>[2x]GSHMPMYEVQWKVVEESNGNNYSYIDPTQLPYDHKWEFPRNRLSFGKTLGAGAFGKVVEATAQGLIKSDAAMTVAVKMLKPSAHSTEREALMSELKVLSYLGNHENIVNLLGACTHGGPTLVITEYCCYGDLLNFLRRKRDEFVPYKVAPEDLYKDFLTLEHLLSFSYQVAKGMAFLASKNCIHRDLAARNILLTHGNITKICDFGLARDIKND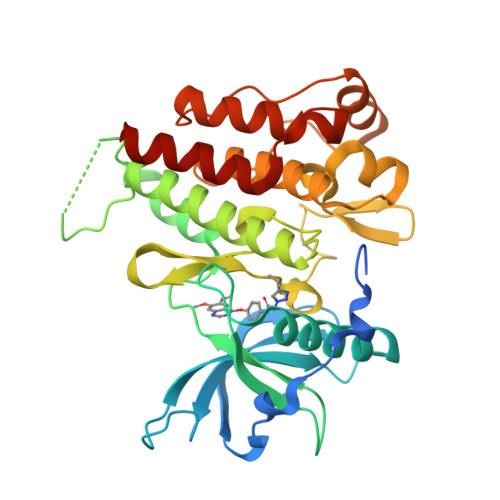SNYVDKGNARLPVKWMAPESIFNSVYTFESDVWSYGIFLWELFSLGSSPYPGMPVDSKFYKMIKEGFRMSSPEYAPAEMYDIMKTCWDADPDKRPTFKQIVQDIEKQISESTNH>[2x]MPRPKLKSDDEVLEAATVVLKRCGPIEFTLSGVAKEVGLSRAALIQRFTNRDTLLVRMMERGVEQVRHYLNAIPIGAGPQGLWEFLQVLVRSMNTRNDFSVNYLISWYELQV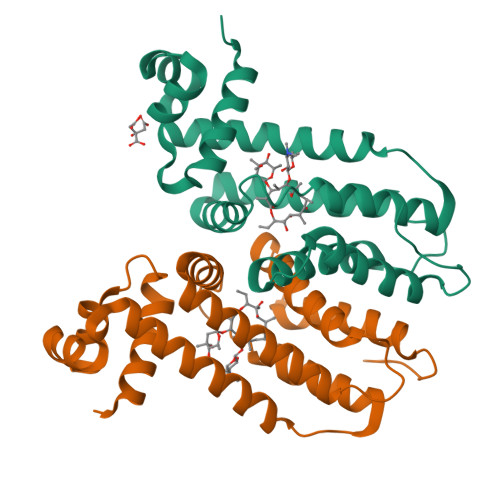PELRTLAIQTNRAVVEGIRNRLPPGAPAAAELLLHSVITGATMQWAVDPDGELADHVLAQIAAILCLMFPEQDDFQLLQAHA>GASQFFKDNCNRTTASLVEGVELTKYISDINNNTDGMYVVSSTGGVWRISRAKDYPDNVMTAEMRKIAXAAVLSGMRVNMCASPASSPNVIWAIELEAE[3x];>GASQFFKDNCNRTTASLVEGVELTKYISDINNNTDGMYVVSSTGGVWRISRAKDYPDNVMTAEMRKIAMAAVLSGMRVNMCASP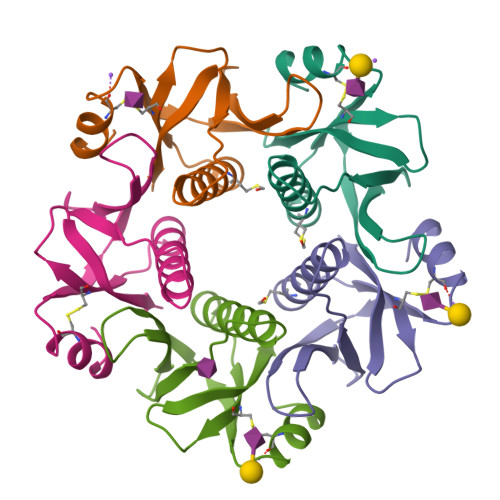ASSPNVIWAIELEAE[2x]> EGTKLDDDFKEMERKVDVTSRAVMEIMTKTIEYLQPNPASRAKPQAEALLAEAMLKFGRELGDDCNFGPALGE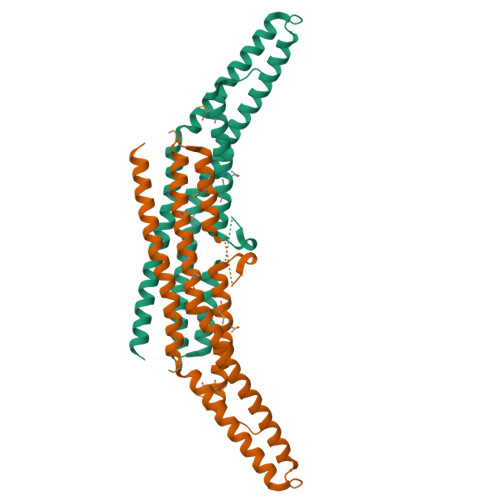VGEAMRELSEVKDSLDMEVKQNFIDPLQNLHDKDLREIQHHLKKLEGRRLDFDYKKKRQGKIPDEELRQALEKFDESKEIAESSMFNLLEMDIEQVSQLSALVQAQLEYHKQAVQILQQVTVRLEERIRQA> GHMTGVESFMTKQDTTGKIISIDTSSL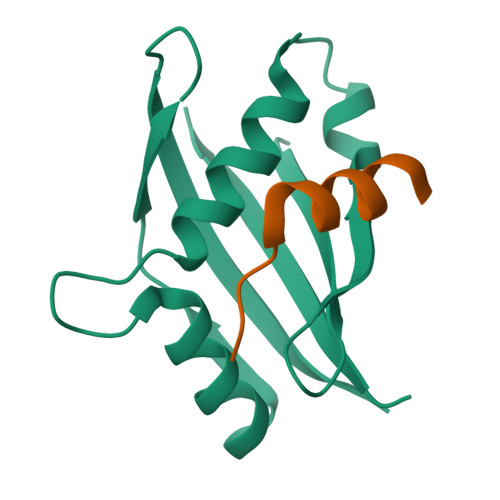RAAGRTGWEDLVRKCIYAFFQPQGREPSYARQLFQEVMTRGTASSPSYRFILNDGTMLSAHTRCKLCYPQSPDMQPFIMGIHIIDREHSGLSPQDDTNSGMSIPR;> GTWIGEDIFPPLLPPTEQDLTKLLLEGQGESG>[4x]SMNSQPFKLDPKSAHRKLKVSHDNLTVERDESSSKKSHTPERFTSQGSYGVAGNVFIDSGRHYWEVVISGSTWYAIGLAYKSAPKHEWIGKNSASWA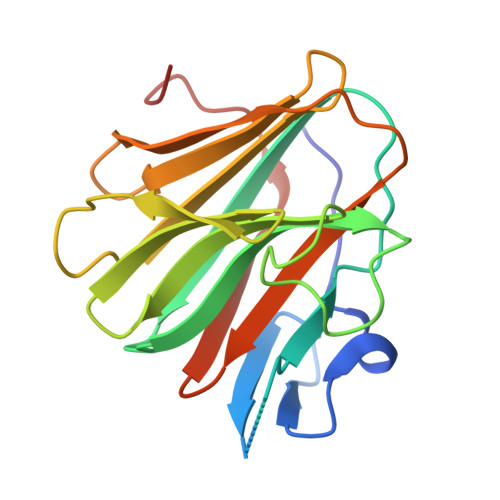LCRCNNNWVVRHNSKEIPIEPAPHLRRVGILLDYDNGSIAFYDALNSIHLYTFDVAFAQPVCPTFTVWNKCLTIITGLPIPDHLDCTEQLP>PSDEAMTVRPVDQRPSLDSTFERLSKLQPTATSCLAKDSESLFNDLCSVFLSAAVSESDLERFDATPVLSRPKAPSNSFYLSFYLRVWCGPYPTLAKVAALERVKTRLKEGDCVDKDFQAIFPYCIAALSDPAKKVRRAAADLVAVLGSAYKSLEKSQQLWAAKDLYGKTGTTSPLDKDALKALIRSVLIPCLEESVLHEDHVVAALVGALESSKDSENKNADKRHLSHSARLSIFKFLCGHVVETPLLAVKLRLLRSLNQIRRISGTTRTDLLLPLLRWWAGLSANEAAELAAQESVDVPAIDDAVVDVVVPNHAAGLEAFFQLVKE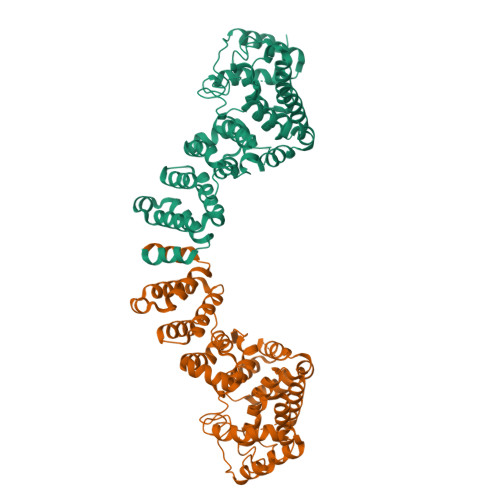AIRPGLLQAIFARIAKMWPSMKSDTKYSTAKTLFELTQDPKLNAEQSDVITEAVEVLRKVDLTTDILHYFIDS[2x]>[3x]GPMGFVPETEDMLPRLAPRPSAAVPMGHTNEIIGPTVPEVSILFGQPPQDKAATPPPAANSSSDFKREITNADGSKDIWYPNGNLKKISADGMNLRMLYFNKDIKETNIREGTVKYYYAETNTWHTSYLDGLEILEFPNGQTEHRRKDGTVEIHFPNNSIKIVDPSDTEKLEEWRYADGTHLVQLRNGDKILNLPNGQKEIHTKLNKRREYPDGTVKLVYPDGSQETRYSNGRVRLKDKDGKLIMDTDYAKY

Of particular interest in this regard is the putative centriolar CPAP–STIL complex, as mutations in both components result in MCPH. CPAP and STIL are strictly required for centriole assembly: STIL at a very early stage and CPAP slightly later, possibly by controlling the organisation and length of the centriolar microtubules. Instead, we demonstrate that the TCP domain of CPAP constitutes a novel proline-rich-motif (PRM) recognition-domain that specifically binds to a short target motif in STIL. Our mutational analysis of the interface demonstrates a remarkable correlation between the ability of mutant proteins to bind to one another in vitro and their ability to support centriole assembly in vivo, providing compelling support for our structural model of the metazoan CPAP–STIL complex. These data strongly suggest that the interaction between CPAP and STIL is a conserved, essential step in centriole biogenesis.

The sequence conservation of the CPAP TCP domain and the CR2 region of STIL suggests that this interaction may be conserved. To confirm this, we solved the crystal structure of the TCP domain from Drosophila melanogaster DSas-4 (dCPAP) (residues 700–901) in complex with the region of Ana2 (dSTIL) equivalent to CR2 (residues 1–47). The dSTIL–dCPAP interaction interface in this structure was highly similar to the D. rerio complex (inter-species alignments of the structures yielded an average pairwise RMSD of 1.2 ± 0.2 Å across an average of 118 ± 4 Cα pairs). Indeed, all copies of the complex obtained in the structures from both species superimposed well and exhibited the same four major groups of binding interactions as described for the D. rerio structure. This conservation includes the contact made by the E792 residue in dCPAP (the equivalent of the E1235 residue in human CPAP that is mutated in MCPH). Although the overall sequence identity of the CPAP and STIL proteins between Drosophila and zebrafish is relatively low (∼22% and ∼13%, respectively), our structural analysis revealed that the interaction interface is conserved, confirming the previous proposal that fly Ana2 is the functional homologue of vertebrate STIL. Despite the many sequence changes between Drosophila Ana2 and vertebrate STIL, our work suggests that the interaction interface between Ana2/STIL and dSAS-4/CPAP TCP domain has been retained, highlighting its importance.>AMYDIYGEAALPADVRERLRITRDLAQAFHERAPEHDRAGDFPFENIEDLKASGYVRWTVPVEYGGLGLSLEEMLMHQEVLAKGDGSTALAIGWHVGILLHLRETGAFPDELFRMVCESVVKEGALINSCATEPATGSPSRGGKPETTAVKVPGGYRITGRKTFSTLSPALTWIMVTATVADEDVVGQFLVRKEDVEIVETWDTLGMRATGSHDIVLKDVFVPEERVIVIQRPGVQAERRPDGSGWLLHIPACYLGIALAARDFALEYAATYRPNTLPHPIAEVPHVEQKLGEMELKLLAARTLLYDLARRFDAASPEERVKLQPQFGAVKTLATNAANQVVDLAMRVVGGRSLSRALPLERYYRDVRAGLHNPPMDDVVYRNLAKAAL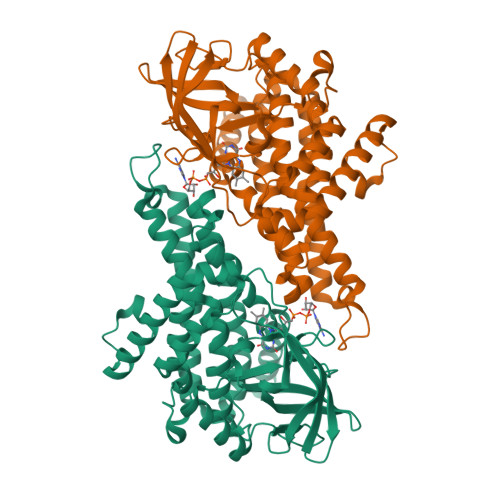ARRAAGQAGR[3x]>[4x]YEHTAVMPNKVGIPYKALVERPGYAPVHLQI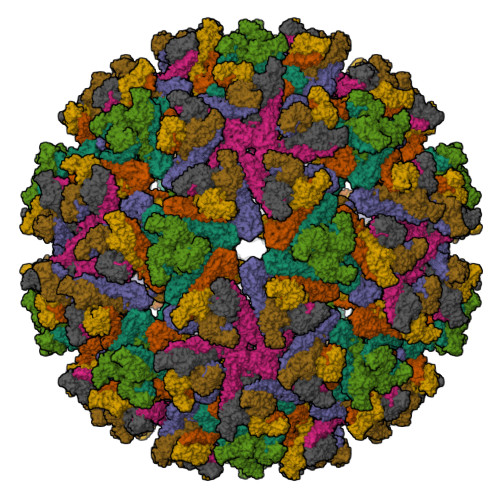QLVNTRIIPSTNLEYITCKYKTKVPSPVVKCCGATQCTSKPHPDYQCQVFTGVYPFMWGGAYCFCDTENTQMSEAYVERSEECSIDHAKAYKVHTGTVQAMVNITYGSVSWRSADVYVNGETPAKIGDAKLIIGPLSSAWSPFDNKVVVYGHEVYNYDFPEYGTGKAGSFGDLQSRTSTSNDLYANTNLKLQRPQAGIVHTPFTQAPSGFERWKRDKGAPLNDVAPFGCSIALEPLRAENCAVGSIPISIDIPDAAFTRISETPTVSDLECKITECTYASDFGGIATVAYKSSKAGNCPIHSPSGVAVIKENDVTLAESGSFTFHFSTANIHPAFKLQVCTSAVTCKGDCKPPKDHIVDYPAQHTESFTSAISATAWSWLKVLVGGTSAFIVLGLIATAVVALVLFFHRH;>DLDTHFTQYKLARPYIADCPNCGHSRCDSPIAIEEVRGDAHAGVIRIQTSAMFGLKTDGVDLAYMSFMNGKTQKSIKIDNLHVRTSAPCSLVSHHGYYILAQCPPGDTVTVGFHDGPNRHTCTVAHKVEFRPVGREKYRHPPEHGVELPCNRYTHKRADQGHYVEMHQPGLVADHSLLSIHSAKVKITVPSGAQVKYYCKCPDVREGITSSDHTTTCTDVKQCRAYLIDNKKWVYNSGRLPRGEGDTFKGKLHVPFVPVKAKCIATLAPEPLVEHKHRTLILHLHPDHPTLLTTRSLGSDANPTRQWIERPTTVNFTVTGEGLEYTWGNHPPKRVWAQESGEGNPHGWPHEVVVYYYNRYPLTTIIGLCTCVAIIMVSCVTSVWLLCRTRNLCITPYKLAPNAQVPILLALLCCIKPTRA[4x]>[4x]MSNATLNQLPGRLGDPSMSLGTDPRTDPRLAAALTQLGLADQAAEPPVNANSEVADCIAYSTAAEQAWQTLGAMLGSQGEPSNPVDVREETIKGRGGNEIKLYIHSPTGHTSDSDPLPCVVHTHGGGMVILTAADANYSRWRSELAATGLVVVGVEFRNAAGALGNHPFPAGLHDCADAAK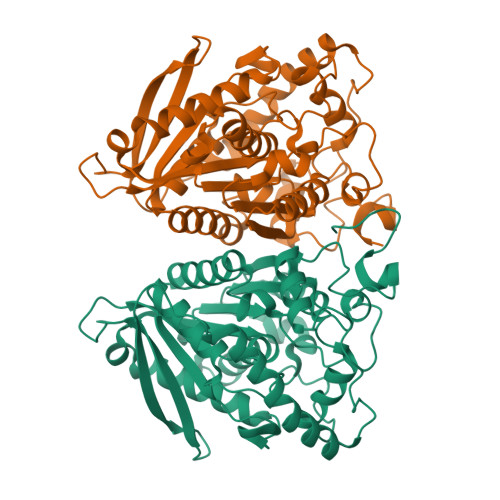WVASNREALGISTLIMSGESGGGNLSLATTMLAKKEGWLEEIAGVYAQCPYISGLYASKPEELPSLLENDAYFWDMKTMGAMVKPYDPTGENASNPLAWPYHASLEDLAGLPPHVISVNELDPLRDEGLAHYRKLLKAGVSTVGRTVHGTCHAADCSFVDVIPDVYFATVRDISAFAYSRA>GHMMKNRIFVSSSKDFEGYPSKAIVPVQFVALLTSIHLTETKCLLGFSNFERRGDQSQEDQYLIKLKFKDRGSERLARITISLLCQYFDIELPDLDSDSGASPTVILRDIHLERLCFSSCKALYVSKHGNYTLFLEDIKPLDLVSVISTISTKST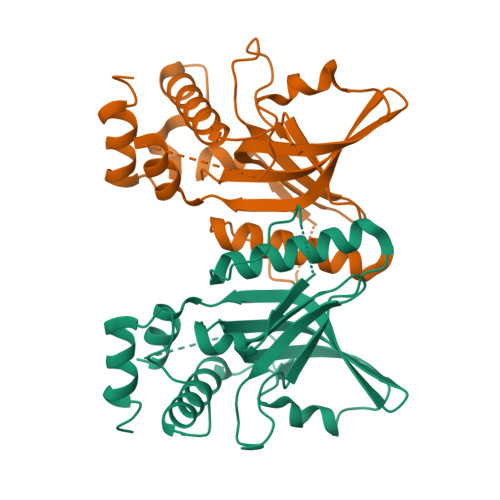NSSKHSSSELISECDLNNSLVDIFNNLIEMNRDEKNRFKFVKLIHYDIELKKFVQDQQKVLSQK[4x]> DVSFRLSGADPS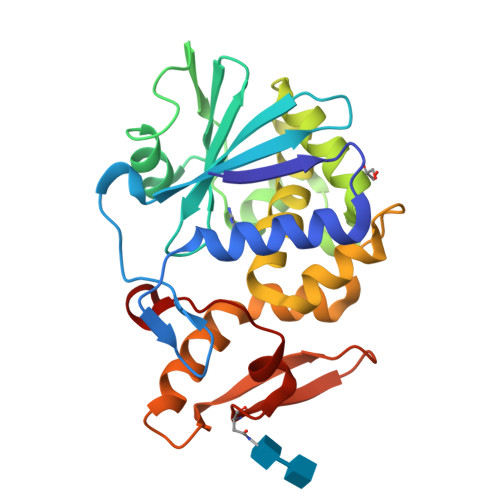SYGMFIKDLRNALPHTEKVYNIPLLLPSVSGAGRYLLMHLFNYDGNTITVAVDVTNVYIMGYLALTTSYFHNEPAADLASQYVFRSARRKITLPYSGNYDRLQIAAGKPREKIPIGLPALDTAISTLLHYDSTAAAGALLVLIQTTAEAARFKYIEQQIQERAYRDEVPSSATISLENSWSGLSKQIQLAQGNNGVFRTPTVLVDSKGNRVQITNVTSNVVTSNIQLLLNTKNI>MAAATGPSFWLGNETLKVPLALFALNRQRLCERLRKNPAVQAGSIVVLQGGEETQRYCTDTGVLFRQESFFHWAFGVTEPGCYGVIDVDTGKSTLFVPRLPASHATWMGKIHSKEHFKEKYAVDDVQYVDEIASVLTSQKPSVLLTLRGVNTDSGSVCREASFDGISKFEVNNTILHPEIVECRVFKTDMELEVLRYTNKISSEAHREVMKAVKVGMKEYELESLFEHYCYSRGGMRHSSYTCICGSGENSAVLHYGHAGAPNDRTIQNGDMCLFDMGGEYYCFASDITCSFPANGKFTADQKAVYEAVLRSSRAVMGAMKPGVWWPDMHRLADRIHLEELAHMGILSGSVDAMVQAHLGAVFMPHGLGHFLGIDVHDVGGYPEGVERIDEPGLRSLRTARHLQPGMVLTVEPGIYFIDHLLDEALADPARASFLNREVLQRFRGFGGVRIEEDVVVTDSGIELLTCVPHTVEEIEACMAGCDKAFTPFSGPK[2x]

Prolidase Deficiency (PD) is an autosomal recessive rare disorder caused by loss or reduction of prolidase enzymatic activity due to variants in the PEPD gene. The PEPD gene encodes the enzyme peptidase D (EC 3.4.13.9), also known as prolidase, which is the only enzyme in humans capable of hydrolysis of dipeptides containing proline (Pro) or hydroxyproline (Hyp) on their C-terminus. Prolidase is particularly important in the degradation of collagens, a family of proteins where proline and hydroxyproline account for up to 22% of the amino acid content. We presented here two high-resolution crystal structures for the p.(Arg470His) variant of human prolidase.

The electron density maps clearly indicated the presence of an imidazol side chain rather than a guanidinum group at amino acid position 470, proving the success of the introduced amino acid substitution. The obtained crystals were transferred to cryo-protectant solution containing 25% (v/v) glycerol in mother liquor supplemented with the ligands of interest (20 mM MnCl2 and 20 mM GlyPro). Despite an apparently unaltered active site architecture, the bound substrate remains intact. This was in contrast to wild-type prolidase, where a substitution of Mn2+ by Mg2+ ions was necessary to capture the substrate-bound state. In hProl, Arg470 was located close to the active site and it formed hydrogen bond/ salt bridges with 3 residues: Thr289, Glu452 and Glu453. Glu452 is part of the active site and it participates in catalysis by coordinating both manganese ions. In case of hProlArg470His, substitution of Arg by His resulted in lesser number of salt bridges. His470 forms interacted only with Thr289 and Glu453. Significantly higher B-factors could be observed also for the GlyPro ligand and one of the Mn2+ ions in the structure of the pathological variant in complex with Mn ions and the GlyPro substrate. It seems that the lack of interaction with the catalytically important Mn-coordinating residue Glu452 could therefore cause flexibilization of the active site.> MAAEEEDEVEWVVESIAGF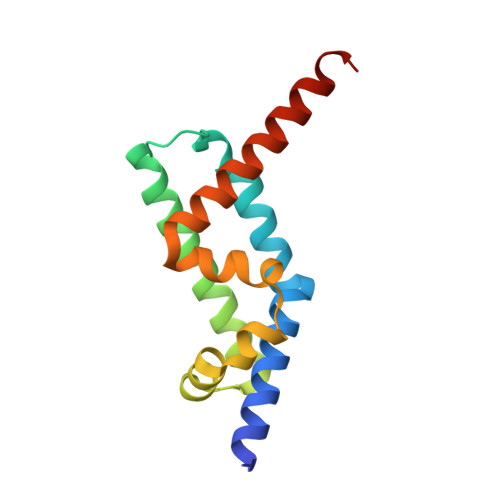LRGPDWSIPILDFVEQKCEVFDDEEESKLTYTEIHQEYKELVEKLLESYLKEIGINEDQFQEACTSPLAKTRTSQAILQPVLAAEDFTIFKAMMVQKNIEMQLQAIRIIQERNG> MGSVTPIPLPKIDEPEEYNTNYILFWNHVGLELNRVTHTVGGPLTGPPLSARALGMLHLAIHDAYFSICPPTDFTTFLSPDTENAAYRLPSPNGANDARQAVAGAALKMLSSLYMKPVEQPNPNPGANISDNAYAQLGLVLDRSVLEAPGGVDRESASFMFGEDVADVFFALLNDPRGASQEGYHPTPGRYKFDDEPTHPVVLIPVDPNNPNGPKMPFRQYHAPFYGKTTKRFATQSEHFLADPPGLRSNADETAEYDDAVRVAIAMGGAQALNSTKRSPWQTAQGLYWAYDGSNLIGTPPRFYNQIVRRIAVTYKKEEDLANSEVNNADFARLFALVDVACTDAGIFSWKEKWEFEFWAPLSGVRDDGRPDHGDPFWLTLGAPATNTNDIPFKPPFPAYPSGHATFGGAVFQMVRRYYNGRVGTWKDDEPDNIAIDMMISEELNGVNRDLRQPYDPTAPIEDQPGIVRTRI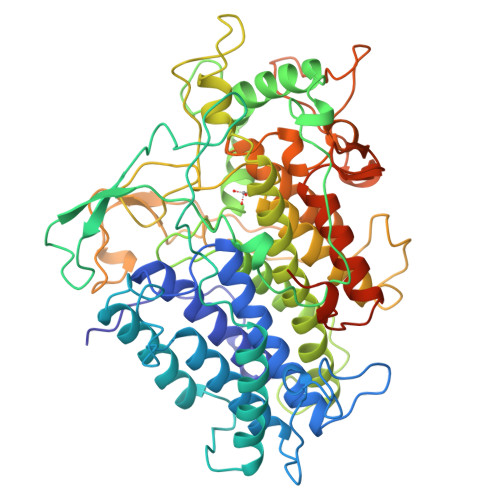VRHFDSAWELMFENAISRIFLGVHWRFDAAAARDILIPTTTKDVYAVDNNGATVFQNVEDIRYTTRGTREDEEGLFPIGGVPLGIEIADEIFNNGLKPTPPEIQPMPQETPVQKPVGQQPVKGMWEEEQAPVVKEAP>[2x]DATWLPPSRWDDGIPGLMLDYNLNGTVSRNYQGGDSHQFSYNGTVG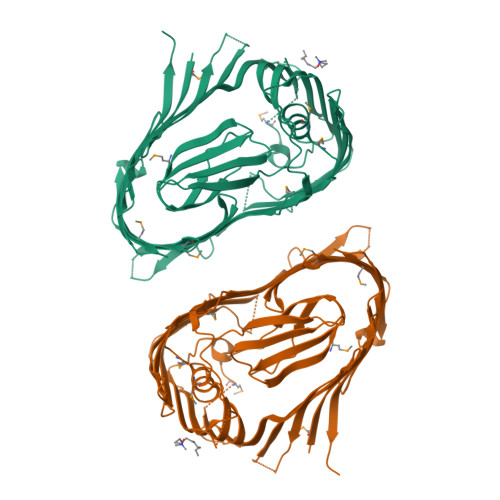GNLGPWRLRADYQGSQEQSRYNGEKTTNRNFTWSRFYLFRAIPRWRANLTLGENNINSDIFRSWSYTGASLESDDRMLPPRLRGYAPQITGIAETNARVVVSQQGRVLYDSMVPAGPFSIQDLDSSVRGRLDVEVIEQNGRKKTFQVDTASVPYLTRPGQVRYKLVSGRSRGYGHETEGPVFATGEASWGLSNQWSLYGGAVLAGDYNALAAGAGWDLGVPGTLSADITQSVARIEGERTFQGKSWRLSYSKRFDNADADITFAGYRFSERNYMTMEQYLNARYRNDYSSREKEMYTVTLNKNVADWNTSFNLQYSRQTYWDIRKTDYYTVSVNRYFNVFGLQGVAVGLSASRSKYLGRDNDSAYLRISVPLGTGTASYSGSMSNDRYVNMAGYTDTFNDGLDSYSLNAGLNSGGGLTSQRQINAYYSHRSPLANLSANIASLQKGYTSFGVSASGGATITGKGALVPR>MASSAQDGNNPLFSPYKMGKFNLSHRVVLAPMTRCRALNNIPQAALGEYYEQRATAGGFLITEGTMISPTSAGFPHVPGIFTKEQVREWKKIVDVVHAKGAVIFCQLWHVGRASHEVYQPAGAAPISSTEKPISNRWRILMPDGTHGIYPKPRAIGTYEISQVVEDYRRSALNAIEAGFDGIEIHGAHGFLIDQFLKDGINDRTDEYGGSLANRCKFITQVVQAVVSAIGADRVGVRVSPAIDHLDAMDSNPLSLGLAVVERLNKIQLHSGSKLAYLHVTQPRYVAYGQTEAGRLGSEEEEARLMRTLRNAYQGTFICSGGYTRELGIEAVAQGDADLVSYGRLFISNPDLVMRIKLNAPLNKYNRKTFYTQDPVVGYTDYPFLQGNGSNGPLSRLLEHHHHHH[2x]

The biocatalytic reduction of the oxime moiety to the corresponding amine group has only recently been found to be a promiscuous activity of ene-reductases transforming α-oximo β-keto esters. By studying the crystal structures of enzyme oxime complexes, analyzing molecular dynamics simulations, and investigating biocatalytic cascades and possible intermediates, we obtained evidence that the reaction proceeds via an imine intermediate and not via the hydroxylamine intermediate. To gain more insight into the reaction pathway, we determined the crystal structures of the two enzymes OPR3 and XenA in complex with the oxime substrates 1a–c, either by co-crystallization or by soaking. All the crystal structures obtained had a high resolution (1.9–1.35 Å) and showed clear electron density features for the oximes.

To assess if the introduced amino acid exchanges affected the overall structure and the binding of the oxime, we also crystallized the tyrosine variants in complex with selected oxime substrates. The protomers in the crystal structures of the tyrosine variants are perfectly superimposable with the ones of the wild-type enzymes, confirming that the exchanges did not lead to major structural alterations. Interestingly, the binding mode of the oxime substrates also did not change in most of the structures. Interestingly, the exchange of the canonical tyrosine (Y190F) did not have an observable effect in this experiment, indicating that fast protonation in the active site is feasible, likely via a water molecule. On the other hand, the canonical tyrosine variant OPR3_Y190F showed a 2-fold increase in kred and an 8-fold decrease for the NADPH Kd. Though a parallel 2-fold increase in kox is also observed, the Kd for the oxime seems not to be affected by the mutation, indicating that the canonical tyrosine residue does not play a role in substrate binding in this enzyme. As an additional aspect of the crystallographic study, the structure of XenA with 1b might explain why only XenA efficiently transformed substrate 1b, and OPR3 did not.>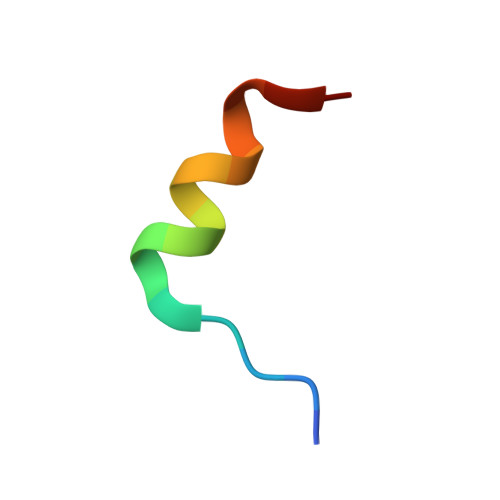 RIIYDRKFLMECRNSPV2-NITRO-P-CRESOL | C7 H7 N O3 | 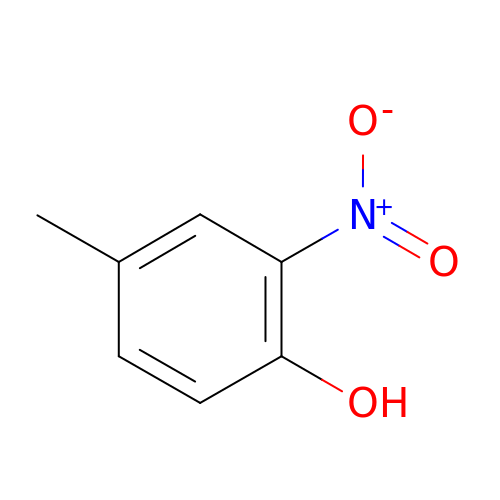SYDNSSSQVSOXTN-UHFFFAOYSA-N> SGRGEA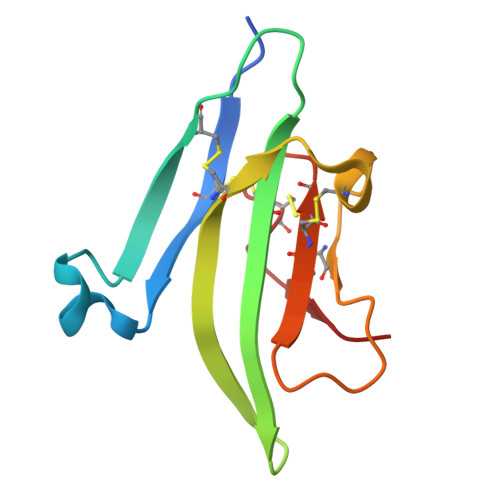ETRECIYYNANWELERTNQSGLERCEGEQDKRLHCYASWRNSSGTIELVKKGCWLDDFNCYDRQECVATEENPQVYFCCCEGNFCNERFTHL> PNPCPESSASFLSRITFWWITGMMVQGYRQPLESTDLWSLNKEDTSEQVVPVLVKNWKKECAKSRKQPVKIVYSSKDPAKPKGSSKVDVNEEAEALIVKCPQKERDPSLFKVLYKTFGPYFLMSFLFKAVHDLMMFAGPEILKLLINFVNDKKAPEWQGYFYTALLFISACLQTLVLHQYFHICFVSGMRIKTAVIGAVYRKALVITNAARKSSTVGEIVNLMSVDAQRFMDLATYINMIWSAPLQVILALYLLWLNLGPSVLAGVAVMVLMVPLNAVMAMKTKTYQVAHMKSKDNRIKLMNEILNGIKVLKLYAWELAFKDKVLAIRQEELKVLKKSAYLAAVGTFTWVCTPFLVALSTFAVYVTVDENNILDAQKAFVSLALFNILRFPLNILPMVISSIVQASVSLKRLRVFLSHEDLDPDSIQRRPIKDAGATNSITVKNATFTWARNDPPTLHGITFSVPEGSLVAVVGQVGCGKSSLLSALLAEMDKVEGHVTVKGSVAYVPQQAWIQNISLRENILFGRQLQERYYKAVVEACALLPDLEILPSGDRTEIGEKGVNLSGGQKQRVSLARAVYCDSDVYLLDDPLSAVDAHVGKHIFENVIGPKGLLKNKTRLLVTHAISYLPQMDVIIVMSGGKISEMGSYQELLARDGAFAEFLRTYASAEQEQGQPEDGLAGVGGPGKEVKQMENGMLVTDTAGKQMQRQLSSSSSYSRDVSQHHTSTAELRKPGPTEETWKLVEADKAQTGQVKLSVYWDYMKAIGLFISFLSIFLFLCNHVASLVSNYWLSLWTDDPIVNGTQEHTQVRLSVYGALGISQGITVFGYSMAVSIGGIFASRRLHLDLLHNVLRSPISFFERTPSGNLVNRFSKELDTVDSMIPQVIKMFMGSLFNVIGACIIILLATPMAAVIIPPLGLIYFFVQRFYVASSRQLKRLESVSRSPVYSHFNETLLGVSVIRAFEEQERFIRQSDLKVDENQKAYYPSIVANRWLAVRLECVGNCIVLFASLFAVISRHSLSAGLVGLSVSYSLQVTTYLNWLVRMSSEMETNIVAVERLKEYSETEKEAPWQIQDMAPPKDWPQVGRVEFRDYGLRYREDLDLVLKHINVTIDGGEKVGIVGRTGAGKSSLTLGLFRIKESAEGEIIIDDINIAKIGLHDLRFKITIIPQDPVLFSGSLRMNLDPFSQYSDEEVWTSLELAHLKGFVSALPDKLNHECAEGGENLSVGQRQLVCLARALLRKTKILVLDEATAAVDLETDDLIQSTIRTQFDDCTVLTIAHRLNTIMDYTRVIVLDKGEIQEWGSPSDLLQQRGLFYSMAKDSGLV;> YFWGNLHWYYEQFDSTCX

pmcMultidrug resistance protein 1 (MRP1) is an ATP-binding cassette (ABC) transporter widely expressed in the lung, kidney, placenta, heart, colon, brain, small intestine, and particularly the blood–brain and blood–testis barriers (1–5). By transporting physiological substrates such as leukotriene C4 (LTC4), MRP1 serves to regulate redox homeostasis, steroid metabolism, inflammation, and hormone secretion. MRP1 is a single polypeptide with five structural domains: an N-terminal transmembrane domain (TMD0) plus a lasso motif (L0), and the canonical ABC transporter architecture of two transmembrane domains (TMD1 and TMD2) and two nucleotide-binding domains (NBD1 and NBD2). Structures of bovine MRP1 (bMRP1) have been determined by cryo-EM in four functional states: an apo (inward-facing) form, an LTC4-bound (inward-facing) form, an ATP-bound (outward-facing) form stabilized by an ATP hydrolysis-defective mutation, and a post-hydrolytic (outward-facing) form. Together, these structures have revealed that MRP1 uses the well-described alternating access mechanism, in which ATP-dependent conformational changes expose the substrate-binding site to alternate sides of the membrane and thereby drive substrate translocation from one side to the other.

CPI1 comprises 17 residues: an N-acylated D-tyrosine (AcDY) followed by 15 proteinogenic amino acids (Phe-Trp-Gly-Asn-Leu-His-Trp-Tyr-Tyr-Glu-Gln-Phe-Asp-Ser-Thr) and a cysteine that forms the thioether linkage with AcDY. A cryo-EM structure of the CPI1–bMRP1 complex in the absence of substrate and ATP was determined to an overall resolution of 3.27 Å. The overall structure of peptide-inhibited MRP1 exhibits an NBD-separated, inward-facing conformation. CPI1 binds at the interface of the two transmembrane helical bundles, filling almost the entire transmembrane pathway. Residues 1 to 13 of CPI are buried at its interface with MRP1, where they engage in extensive hydrogen bonds and van der Waals interactions. The superposition of the CPI1-bound MRP1 structure with the LTC4-bound structure shows that CPI1 binds to the same site as LTC4 and interacts with many of the same residues. CPI1 interacts with residues in both the P- and H-pockets and, because of its large size, engages additional residues toward the cytoplasmic opening of the transmembrane pathway. The solvent-accessible surface area of MRP1 that is buried by CPI1 is 1,580 Å2, about two times that of the binding surface of LTC4 (796 Å2). Because of its large size, CPI1 sterically obstructs the large conformational changes that are required for reorientation of the translocation pathway to an outward-facing conformation. In this manner, CPI1 traps the transporter in an inward-facing, ATPase incompetent state.> GMATGLGEPVY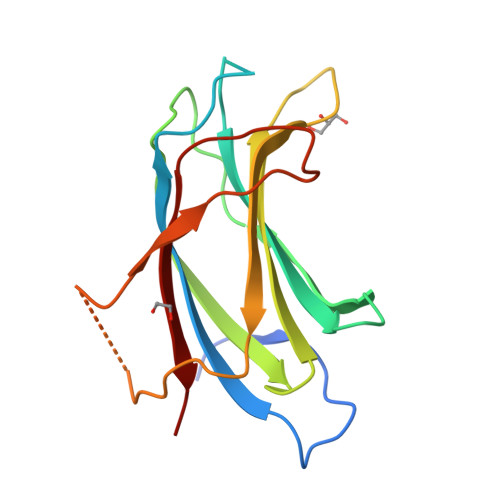GLSEDEGESRILRVKVVSGIDLAKKDIFGASDPYVKLSLYVADENRELALVQTKTIKKTLNPKWNEEFYFRVNPSNHRLLFEVFDENRLTRDDFLGQVDVPLSHLPTEDPTMERPYTFKDFLLRPRSHKSRVKGFLRLKMAYMP> MTVVGAVLPELKLYGDPTFIVSTALATRDFQDVHHDRDKAVAQGSKDIFVNILTDTGLVQRYVTD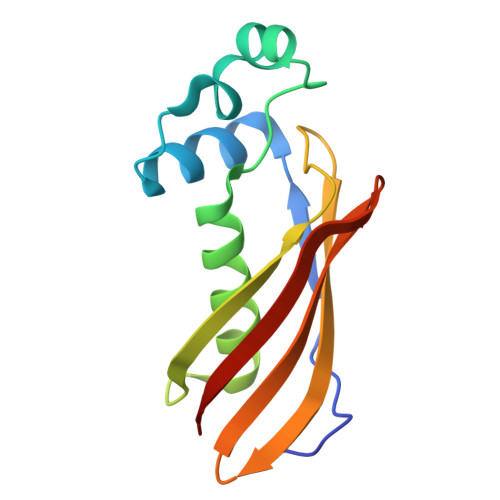WAGPSALIKSIGLRLGVPWYAYDTVTFSGEVTAVNDGLITVKVVGRNTLGDHVTATVELSMRDS>MSKVLVLKSSILAGYSQSGQLTDYFIEQWREKHVADEITVRDLAANPVPVLDGELVGAMRPGDAPLTPRQQDALALSDELIAELKAHDVIVIAAPMYNFNIPTQLKNYFDLIARAGITFRYTEKGPEGLVTGKRAVVLSSRGGIHKDTPTDLIAPYLKVFLGFIGITDVNFVFAEGIAYGPEVAAKAQADAKAAIDSVVAA[2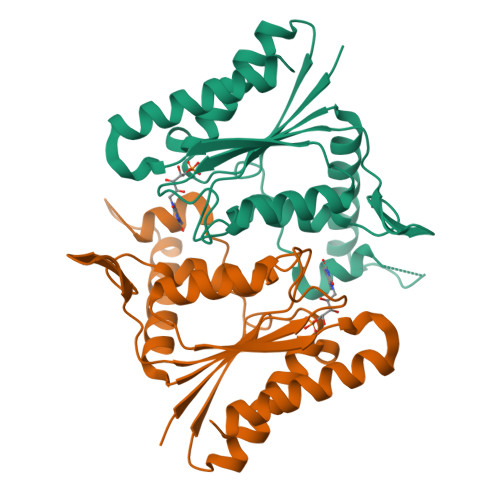x]> XV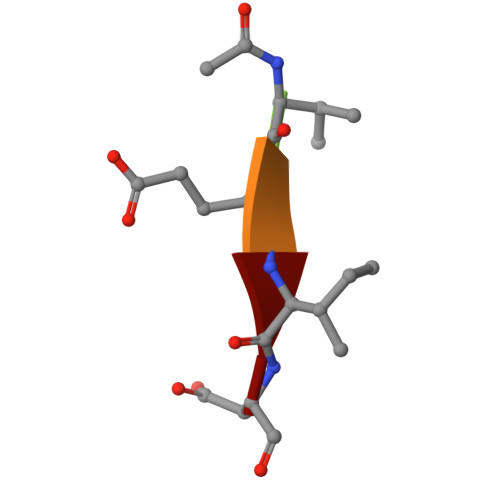EID>SNAMIRKYRYGAPFDTEALTEKIETAEEAFPYGEISQKEGFAFTYIMDEDDIVYGLGESNRGINKRGYCYISNCTDDPIHTEDKRSLYGAHNFIIVSGKTTFGLFFDYPSKLTFDIGYTRMDTLKVSCENADLDIYVIEGENAYDIVKQFRRVIGRSYIPPKFAFGFGQSRWGYTTKEDFRAVAKGYRENHIPIDMIYMDIDYMQDFKDFTVNEKNFPDFPEFVKEMKDQELRLIPIIDAGVKVEKG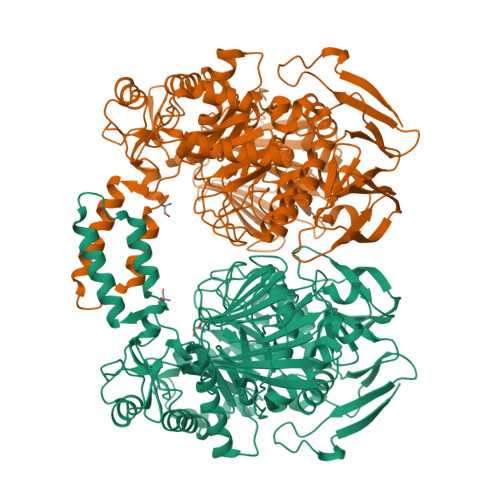YEVYEEGVKNNYFCKREDGSDFVAAVWPGDTHFPDMLNPEARKWFGDKYRFLIDQGIEGFWNDMNEPAIFYSSEGLAEAKEFAGEFAKDTEGKIHPWAMQAKMKDIVNSPEDYKRFYHNVNGKKIRHDKVHNLFGYNMTRAAGEAFERIDPEKRFLMFSRSSYIGMHRYGGIWMGANKSWWSHILLNLKMLPSLNMCGFMYTGADLGGFGDDTTRDLLLRFLALGVFTPLMRDHAAEGTREQECYQFENIEDFRSVINARYRLVPYLYSEYMKAALNDDMYFKPLGFVYPDDKMAIRVEDQLMLGNEIMIAPVYEQNARGRYVYLPEEMKFIKFMPDGSISEEVLEKGVHYVDVALNEVPLFIRSGKCIPVAEAAECVKDIDTENMQLIGYEGSSYTLYEDDGIHKDYDKKENYRVLTK[2x]> SFDCGKPQVEPKKCPGRVVGGCVAHPHSWPWQVSLRTRFGMHFCGGTLISPEWVLTAAHCLEKSPRPSSYKVILGAHQEVNLEPHVQEIEVSRLFLEPTRKDIALLKLSSPAVITDKVIPACLPSPNYVVADRTECFITGWGETQGTFGAGLLKEAQLPVIENKVCNRYEFLNGRVQSTELCAGHLAGGTDSCQGDSGGPLVCFEKDKYILQGVTSWGLGCARPNKPGVYVRVSRFVTWIEGV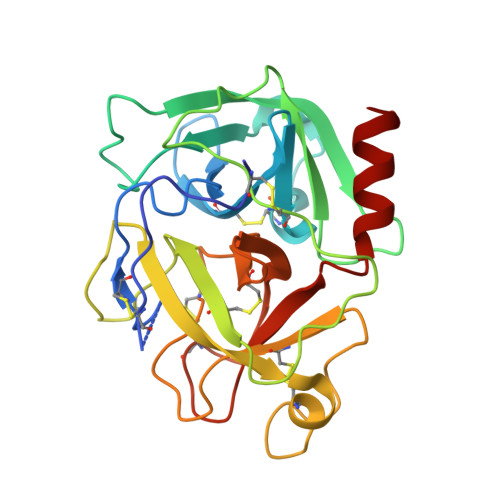MRNN> 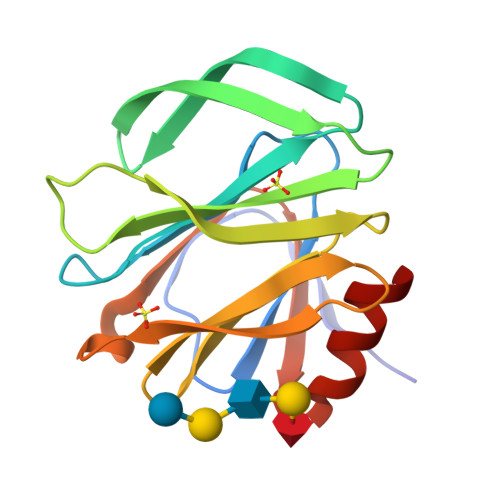GSLDGPYQSTSFKPPSDYWILLNPTNQQVVLEGTNKTDIWVALLLVEPNVTNQSRQYTLFGETKQITVENNTNKWKFFEMFRSSVSAEFQHKRTLTSDTKLAGFLKHYNSVWTFHGETPHATTDYSSTSNLSEVETTIHVEFYIIPRSQESKCVEYINTGL D-ribulose | C5 H10 O5 | 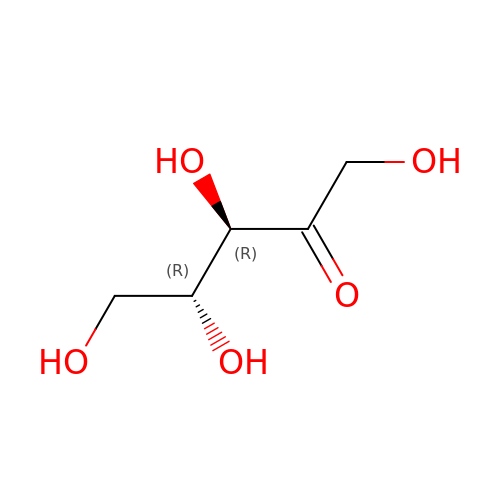ZAQJHHRNXZUBTE-NQXXGFSBSA-N> RDYILAPARPDKLVVIDTEKMAVDKVITIADAGPTPMVPMVAPGGRIAYATVNKSESLVKIDLVTGETLGRIDLSTPEERVKSLFGAALSPDGKTLAIYESPVRLELTHFEVQPTRVALYDAETLSRRKAFEAPRQITMLAWARDGSKLYGLGRDLHVMDPEAGTLVEDKPIQSWEAETYAQPDVLAVWNQHESSGVMATPFYTARKDIDPADPTAYRTGLLTMDLETGEMAMREVRIMDVFYFSTAVNPAKTRAFGAYNVLESFDLEKNASIKRVPLPHSYYSVNVSTDGSTVWLGGALGDLAAYDAETLEKKGQVDLPGNASMSLASVRLF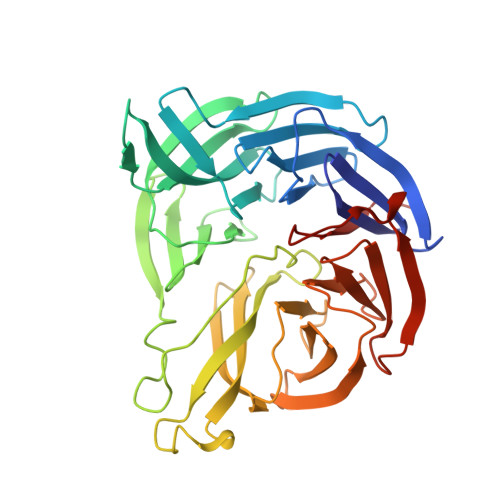TRDE1-(5-chloro-2,4-dimethoxyphenyl)-3-pyrazin-2-ylurea | C13 H13 Cl N4 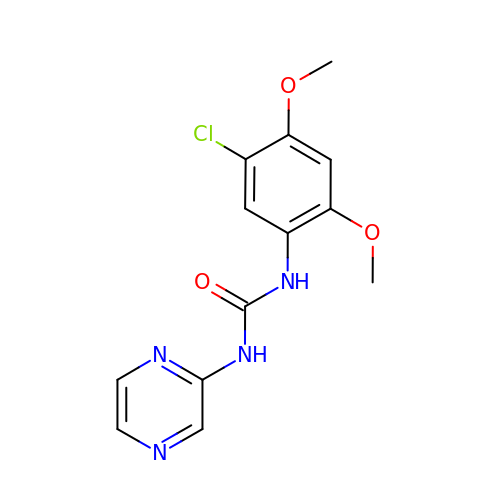O3 | YHZULYLGPVGRKP-UHFFFAOYSA-N> MAQETYFYGQGEIDAAPIVNGVLGKWRWIQDVSAMSIQLAVEKVEHKESYSGQKALVRSFPIGKT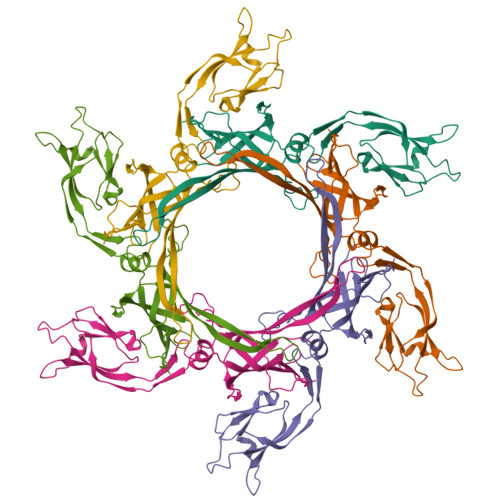ATVNITLHSIGPDNLALTLYGKVVAKAAGSVTGEVLPADLVAGDVIRLANFGVSELVITDSASSPAPLDPQYYALRADGAYGEVQLLGLPTPAPTQPFKAAYEYAATKQVGMFTAPQPTVALRYKGINLAEGGAPVIVELYKVATDPLQELALISDGNTVAGMQISGGILLDTSKPDTGDLGRFGRIIQLG>GPGSPAASKSDKLAATPGMFVQHSTAAFSDRYKGQRVLGKGSFGEVILCKDKVTGQEYAVKVISKRQVKQKTDKELLLKEVELLKKLDHPNIMKLYEFFEDKGYFYLVTEVYTGGELFDEIISRKRFSEVDAARIIRQVLSGITYMHKNKIVHRDLKPENLLLENKRKDANIRIIDFGLSTHFESTKKMKDKIGTAYYIAPEVLHGTYDEKCDVWSTGVILYILLSGCPPFNGANEFDILKKVEKGKFTFDLPQWKKVSEPAKDLIRKMLAYVPTMRISARDALEHEWLKTTDAATDSIDVPSLESTILNI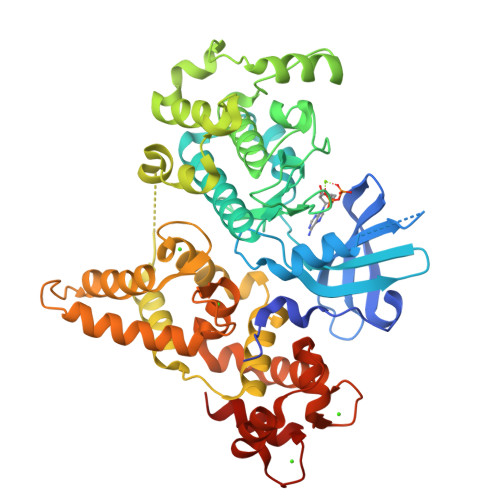RQFQGTQKLAAAALLYMGSKLTTNEETVELNKIFQRMDKNGDGQLDKQELMEGYVELMKLKGEDVSALDQSAIEFEVEQVLDAVDFDKNGFIEYSEFVTVAMDRKTLLSRQRLERAFGMFDADGSGKISSSELATIFGVSEVDSETWRRVLAEVDRNNDGEVDFEEFRQMLLKLCGDTAA[2x]Copper-dependent lytic polysaccharide monooxygenases (LPMOs) classified in Auxiliary Activity (AA) families are considered indispensable as synergistic partners for cellulolytic enzymes to saccharify recalcitrant lignocellulosic plant biomass. In this study, we characterized two fungal oxidoreductases from the new AA16 family. We found that MtAA16A from Myceliophthora thermophila and AnAA16A from Aspergillus nidulans did not catalyze the oxidative cleavage of oligo- and polysaccharides. Further, we showed that both AA16 proteins are able to oxidize low-molecular-weight reductants to produce H2O2.

The three-dimensional structure of MtAA16A, the first experimental structure in the AA16 family, shows the typical LPMO fold. A search with DALI55,56 revealed high structural similarity with AA9, AA10, and AA11 family members, but MtAA16A has a significantly smaller size than the matched structures (see Figure S5 for comparison). The copper binding site appears to be identical to the one observed in AA9, AA11, AA13, AA15, AA17, and some AA10 members with the His-brace providing three equatorial ligands and an additional Tyr axial ligand with typical distances from the copper to the N ligands (1.8–2.3 Å) and a longer distance to the Tyr–OH (2.7 Å). The methylation of His1 is confirmed in the structure. In the crystal, a carboxylic residue from a neighboring molecule blocks the equatorial position to the copper, expecting to bind water in solution. There is no visible axial ligand, presumably due to photoreduction of the Cu(II) to Cu(I) under X-ray exposure. Second coordination sphere residues include a Gln, which is in the same position as an important and conserved Gln in AA9,57 while the conserved second coordination sphere His from AA9 is substituted by an Asn. The surface adjacent to the His-brace in MtAA16A lacks the typical flat aromatic features seen in most cellulose-binding LPMOs and exemplified in the complex of LsAA9A with cellohexaose by interaction with a Tyr. At the surface of MtAA16A, another Tyr residue (Tyr27) can be found near the His-brace but lies sideways rather than parallel to the protein surface. Thus, MtAA16A does not seem to possess a likely polysaccharide-binding surface adjacent to the His-brace but rather a small pocket, which could be speculated to interact with small aromatics like syringol, on which we have demonstrated activity.

>MAKTLFRLVSFAAALSTVLGHAVVTVPTPRGAGPYYTQRCGETYAVYMEKDKAGPIENGVAKAGSELGCNPFLCRGYQYEDNEAVEYEPGQVIDFHVDLIAGHHPGYANVSIVDLEANKIIGDPLRSWDDYPNATATTPRSDIDFNVTIPNTLGTACSTGGKCAIQWYWYASGNKQSYESCVDFYVKA[3x]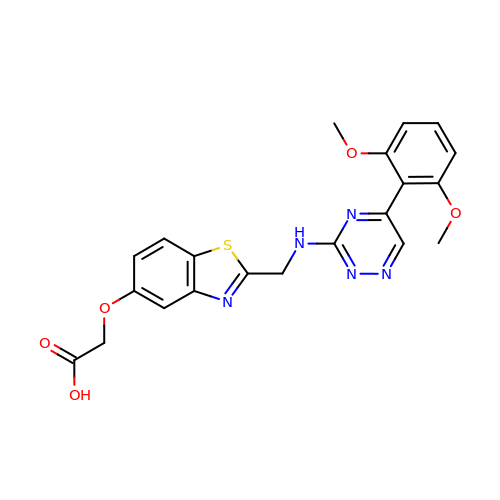{[2-({[5-(2,6-dimethoxyphenyl)-1,2,4-triazin-3-yl]amino}methyl)-1,3-benzothiazol-5-yl]oxy}acetic acid | C21 H19 N5 O5 S | CNAYNNSUTSXUJE-UHFFFAOYSA-N ethyl 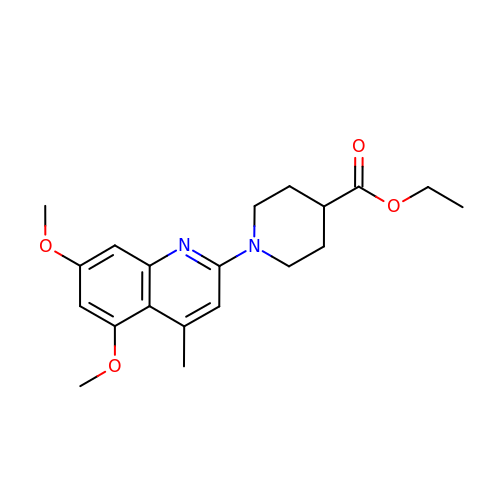1-(5,7-dimethoxy-4-methylquinolin-2-yl)piperidine-4-carboxylate | C20 H26 N2 O4 | QMSAXOQPCCJWDP-UHFFFAOYSA-N>[12x]MAPITAYSQQTRGLLGCIITSLTGRDRNQVEGEVQVVSTATQSFLATCV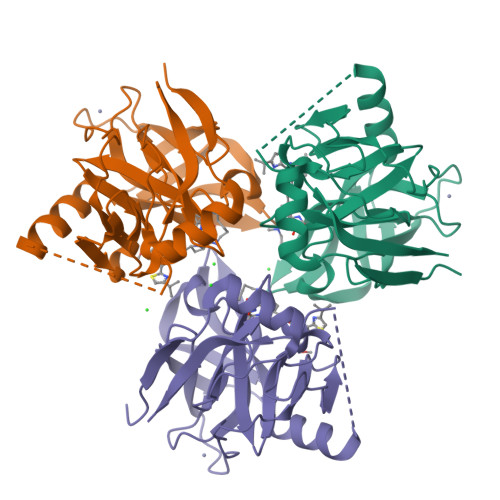NGVCWTVYHGAGSKTLAGPKGPITQMYTNVDQDLVGWQAPPGARSLTPCTCGSSDLYLVTRHADVIPVRRRGDSRGSLLSPRPVSYLKGSSGGPLLCPSGHAVGIFRAAVCTRGVAKAVDFVPVESMETTMRASKKKKKGSVVIVGRIILSGRK> IKTVLDTAQAPYKGSTVIGHALSKHAGRHPEIWGKVKGSMSGWNEQAMKHFKEIVRAPGEFRPTMNEKGITFLEKRLIDGRGVRLNLDGTFKGFID;> MKELFEVIFEGVNTSRLFFLLKEIESKSDRIFDFNFSEDFFSSNVNVFSELLIDSFLGFNGDLYFGVSMEGFSVKDGLKLPVVLLRVLKYEGGVDVGLCFYMNDFNSAGKVMLEFQKYMNGISADFGFENFYGGLEPASDQET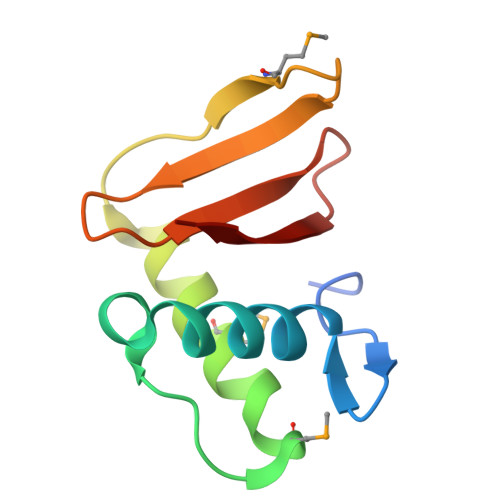RFFTNNRLGPLL N,N'-bis(1-methylethyl)phosphorodiamidic acid | C6 H17 N2 O2 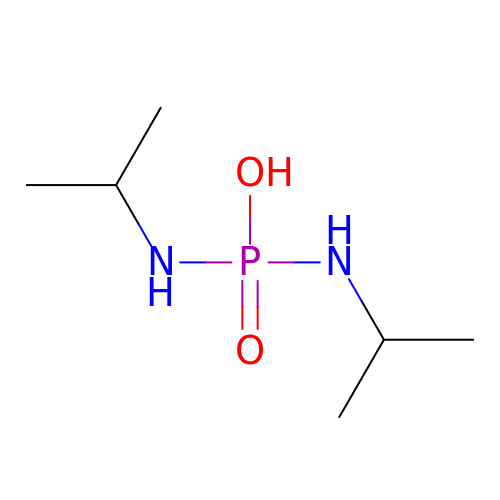P | CAMCMEOOLQEXTO-UHFFFAOYSA-N> FSVLNWDQVSRLHEVLTEVVPIHGRGNFPTLEITLKDIVQTVRSRLEEAGIKVHDVRLNGSAAGHVLVKDNGLGCKDLDLIFHVALPTEAE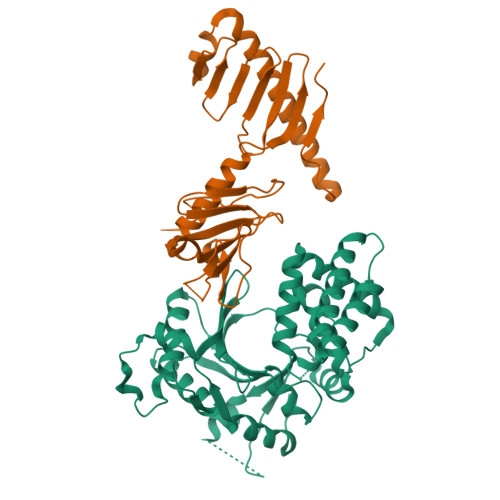FQLVRDVVLCSLLNFLPEGVNKLKISPVTLKEAYVQKLVKVCTDTDRWSLISLSNKNGKNVQLKFVDSIRRQFEFSVDSFQIILDSLLDFYDCSNNPISEHDHPTVIGESMYGDFEEAFDHLQNRLIATKNPEEIRGGGLLKYSNLLVRDFRPTDQEEIKTLERYMCSRFFIDFPDILEQQRKLETYLQNHFAEEERSKYDYLMILRRVVNESTVCLMGHERRQTLNLISLLALRVLAEQNIIPSATNVTCYYQ;> RTLRSITSPLVAHRLKPIRQKTKKAVVSILDSEEVCVELVKEYASQEYVKEVLQISSDGNTITIYYPNGGRGFPLADRPPSPTDNISRYSFDNLPEKYWRKYQYASRFVQLVRSKSPKITYFTRYAKCILMENSPGADFEVWFYDGVKIHKTEDFIQVIEKTGKSYTLKSESEVNSLKEEIKMYMDHANEGHRICLALESIISEEERKTRSAPFFPIIIGRKP> SMGLLQLLSNGTVLRSESIDLITQQIPFKNNQTVLFKDSIYHKPNNLHLRLYKPISASNRTALPVVVFFHGGGFCFGSRSWPHFHNFCLTLASSLNALVVSPDYRLAPEHRLPAAFEDAEAVLTWLWDQAVSDGVNHWFEDGTDVDFDRVFVVGDSSGGNIAHQLAVRFGSGSIELTPVRVRGYVLMGPFFGGEERTNSENGPSEALLSLDLLDKFWRLSLPNGATRDHHMANPFGPTSPTL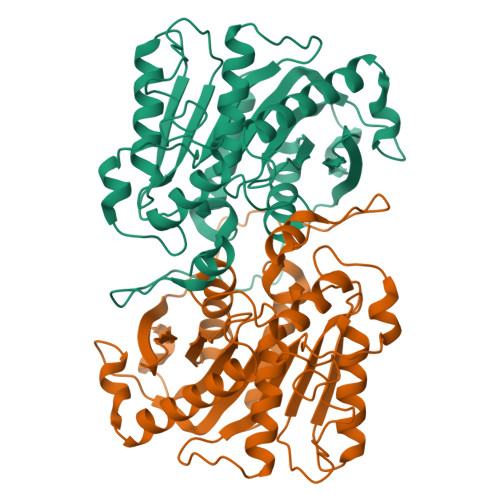ESISLEPMLVIVGGSELLRDRAKEYAYKLKKMGGKRVDYIEFENKEHGFYSNYPSSEAAEQVLRIIGDFMNNLS Mitochondrial Hsp60 (mtHsp60) plays a crucial role in maintaining the proper folding of proteins in the mitochondria. mtHsp60 self-assembles into a ring-shaped heptamer, which can further form a double-ring tetradecamer in the presence of ATP and mtHsp10. The crystal structure of mtHsp60 reveals three domains: apical, intermediate, and equatorial domains. The equatorial domain connects the subunits in the heptameric ring and facilitates interactions between the two rings of tetradecamers. Our results showed that the E. coioides mtHsp60 (EcHsp60) forms dimers that are incapable of hydrolyzing ATP but can reassemble into heptamers, thus restoring ATPase activity.

To understand the molecular basis of the inactivation of dimeric EcHsp60, the crystal structure of the naïve EcHsp602 was solved at a resolution of 2.35 Å. The dimeric structure of the naïve EcHsp60 (EcHsp602) revealed a twofold symmetrical conformation, with two protomers facing each other in an asymmetric unit. The N-terminal (MIS and residues 1–87) and the C-terminal (residues 508–552) regions of both protomers were not observed in the density maps because of their disordered structure, and only a partial equatorial domain was built in this model. The equatorial domain of the naïve EcHsp602 showed greater flexibility compared with the apical domain, as indicated by a higher average b-factor. The α4 helix of each subunit protruded out from its equatorial domain to interact with the adjacent subunit, with the interface mainly composed of van der Waals forces and hydrophobic interactions. Two intermolecular polar contacts were identified on the α4 helix of each subunit, involving residues T89, E100, D103, R444, and D494. The RLK motif (R264-K266) located at the α9 terminus formed four hydrogen bonds with residues from another protomer, including E212, R264, L265, and K266. The T89 forms hydrogen bonds with D494, occupying the space of the ATP-binding pocket, and the D85, G86, and T87 are disordered, leading to the inability of EcHsp602 to hydrolyze ATP. In contrast, neither the naïve nor the mature EcHsp602 showed any ATP hydrolysis activity at any ATP concentration. The oligomeric conformation of the R264AK266A mutant was confirmed by negative-stain TEM, which showed that it formed a heptameric ring structure similar to the WT naïve EcHsp607. These results suggest that the RLK motif is crucial for stabilizing the dimeric form of EcHsp60.

>MFRLPTVMKQVRPVCRALAPHLTRAYAKDVKFGADARALMLQGVDLLADAVAVTMGPKGRTVIIEQSWGSPKVTKDGVTVAKSIDLKDKYKNIGAKLVQDVANNTNEEAGDGTTTATVLARAIAKEGFDTISKGANPVEIRRGVMMAVETVIKELKNLSKPVTTPEEIAQVATISANGDVEIGNIISNAMKKVGRKGVITVKDGKTLHDELEIIEGMKFDRGYISPYFINTAKGQKCEFQDAYLLLSEKKISSVQSIVPALEIANQHRKPLVIVAEDVDGEALSTLVLNRLKVGLQVVAVKAPGFGDNRKNQLRDMAVATGGTVFGDEAVGLALEDIQAHDFGKIGEVQITKDDTLLLKGGGSPAEVEKRAAEIVEQLENTTSDYEKEKLNERLAKLSDGVAVLKVGGTSDVEVNEKKDRVTDALNATRAAVEEGIVPGGGCALLRCIPSLDAIQTANADQKIGVEIIRRALRIPAMTIAKNAGVEGSLVVEKILQGSAELGYDAMQGEYVNMVEKGIIDPTKVVRTALLDAAGVASLLSTAEAVVTEIPKEEKEMPGGMGGMGGMGGMGGMGGGMGFLEHHHHHH[2x]>MSSHHHHHHSSGLVPRGSHMTDQGLEGSNPVDLSKHPSGIVPTLQNIVSTVNLDCKLDLKAIALQARNAEYNPKRFAAVIMRIREPKTTALIFASGKMVCTGAKSEDFSKMAARKYARIVQKLGFPAKFKDFKIQNIVGS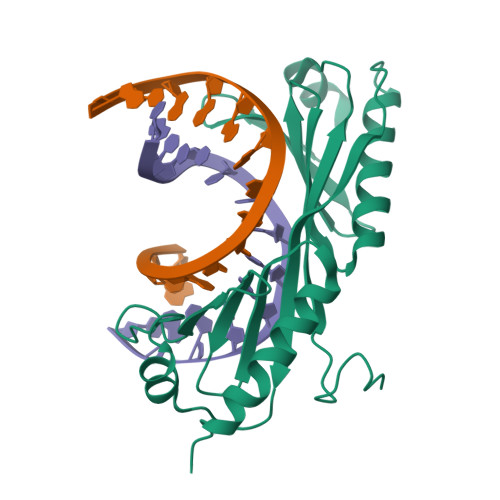CDVKFPIRLEGLAYSHAAFSSYEPELFPGLIYRMKVPKIVLLIFVSGKIVITGAKMRDETYKAFENIYPVLSEFRKIQQ[4x]> MIRRAPTTLQLSHDDVTSLIDDLNEQKLKQQLNIEKTKYFQGKNGGSLHSNTDFQDTSQNIEDNNNDNDNDIDED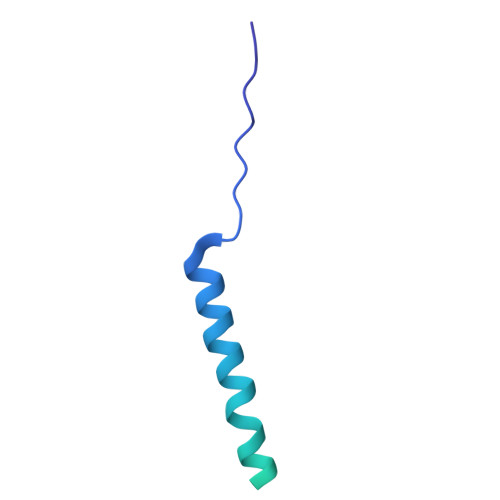DDMSSYNDKAASVAHTRVLNSLHLSTDSNTAHETSNANDNHNPFYIREE>SDENDTARKIIKTLLDIMREGDEDKLRDQMDPNVRADVGDKTVHGREHAAKFLAHIVKRADHISFTLKSLHNHNGRLRMQGEVRIVHNGRTERVPLE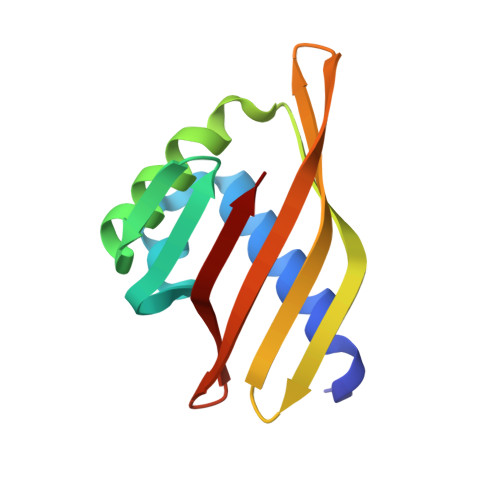MVFRKHNGKWLIERMKYG[2x]>[2x]MVPSYDSFDYEDYPAALPNHKPKGTFKDYVRDRADLNKDKPVIPAAALAGYTGSGPIQLWQFLLELLTDKSCQSFISWTGDGWEFKLSDPDEVARRWGKRKNKPKMNYEKLSRGLRYYYDKNIIHKTAGKRYVYRFVCDLQSLLGYTPEELHAMLDVKPDADE

Ets1, a founding member of the Ets (E-twenty-six-specific) family of transcription factors, was initially identified as the protooncogene corresponding to v-ets of the E26 leukemia virus. Ets1 regulates expression of lymphocyte-specific genes, bone-specific genes, and genes involved in vascular development and angiogenesis. Ets family members contain a highly conserved DNA-binding Ets domain, an 85-amino acid winged helix-turn-helix DNA-binding domain which recognizes a core motif 5′-GGA(A/T)-3′ referred to as Ets-binding site (EBS). In the case of Ets1, autoinhibition is mediated by structural coupling of the regions flanking the DNA-binding domain.

To verify Ets1 dimer binding to two separate pieces of DNA we crystallized and solved the structure of the complex comprised of Ets1 dimer and two pieces of DNA [referred to as (Ets1)2•2DNA]. The asymmetric unit contains two Ets1 molecules (residues 280–441) forming a dimer. The DNA-binding areas of each Ets1 subunit are on the same side of the dimer and docked on two antiparallel pieces of dsDNA from TCRα promoter. Each Ets1 is bound to a separate piece of dsDNA resulting in formation of (Ets1)2•2DNA quaternary complex. The structure revealed that in spite of DNA binding the overall conformation of Ets1 dimer, including HI1 and HI2, remains the same. Briefly, at each position the interactions involve the N-terminal portion of HI1 helix from one subunit and H4 helix, a loop H4H5, HI2 helix and a loop HI1HI2 from another subunit. However, within (Ets1)2•2DNA complex additional hydrogen bonds are observed between each Ets1 subunit and the neighboring DNA duplex. The potential hydrogen bonds involve the side chains of Asn380 and Lys383 from the loop H2H3 and DNA phosphate oxygen. Superimposition of Ets1 dimers with and without DNA shows that DNA binding introduces only minor local changes in Ets1 dimer structure with the root-mean-square deviations for the 271 matched α-carbon atoms at 0.86 Å. The only notable difference is the disorder of the seven N-terminal residues within (Ets1)2•2DNA complex.>[2x]SQAARVDYIAPWWVVWLHSVPHVGLRLQPVNSTFSPGDESYQESLLFLGLVAAVCLGLNLIFLVAYLVCACHCRRDDAVQTKQHHSCCITWTAVVAGLICCAAVGVGFYGNSETNDGAYQLMYSLDDANHTFSGIDALVSGTTQKMKVDLEQHLARLSEIFAARGDYLQTLKFIQQMAGSVVVQLSGLPVWREVTMELTKLSDQTGYVEYYRWLSYLLLFILDLVICLIACLGLAKRSKCLLASMLCCGALSLLLSWASLAADGSAAVATSDFCVAPDTFILNVTEGQISTEVTRYYLYCSQSGSSPFQQTLTTFQRALTTMQIQVAGLLQFAVPLFSTAEEDLLAIQLLLNSSESSLHQLTAMVDCRGLHKDYLDALAGICYDGLQGLLYLGLFSFLAALAFSTMICAGPRAWKHFTTRNRDYDDIDDDDPFNPQAWRMAAHSPPRGQLHSFCSYSSGLGSQTSLQPPAQTISNAPVSEYMNQAMLFGRNPRYENVPLIGRASPPPTYSPSMRATYLSVADEHLRHYGNQFPAALEVLFQ

The Tweety homologs (TTYHs) are members of a conserved family of eukaryotic membrane proteins that are abundant in the brain. The three human paralogs were assigned to function as anion channels that are either activated by Ca2+ or cell swelling. All TTYH molecules are dimers and contain an extended extracellular domain, five membrane spanning segments, and an unstructured cytoplasmic region. In light of its distinct protein architecture and the absence of functional evidence for ion transport, we thus conclude that the TTYH family does not form ion channels and instead confers other catalytic properties.

To obtain a comprehensive overview of TTYH conformations, we have investigated the structural properties of all three paralogs in distinct environments: The structures of TTYH2 and 1 were determined in GDN under Ca2+-free conditions at 3.3 and 4.0 Å, respectively. Both proteins display a novel fold with very similar general features. For simplicity, we describe these common features based on the TTYH2 structure and emphasize differences to other paralogs wherever relevant. In TTYH2, the interactions between subunits are exclusively mediated by this extracellular component, which buries 1800 Å2 of the combined molecular surface in an extended dimer interface. Whereas in both structures of TTYH2 determined in detergent and in lipid nanodiscs, the two transmembrane domains (TMDs) are separated by about 7 Å and thus not in direct contact, they have approached each other in the TTYH1 and 3 structures by mutual rigid body rotations of subunits by 6–7° around an axis located at the extracellular dimer interface. Additionally, there are contacts between the TMDs of TTYH1 and 3 but not of TTYH2. In cryo-EM maps of the three paralogs obtained in detergent, the pocket is filled with residual density reflecting its occupancy by small molecules. In TTYH2, six elongated density fragments line the entire pocket perpendicular to its long dimension. As all proteins were purified in the detergent GDN, we cannot exclude that the observed density would reflect the interaction with its cholesterol-derived diosgenin moiety or breakdown products thereof. To investigate the apolar content of molecules that are co-purified with TTYH2, we have prepared methanol and chloroform extracts of a purified sample and analyzed its composition by liquid chromatography and mass spectrometry (LC-MS).> MREDTKVYDITIIGGGPVGLFTAFYGGMRQASVKIIESLPQLGGQLSALYPEKYIYDVAGFPKIRA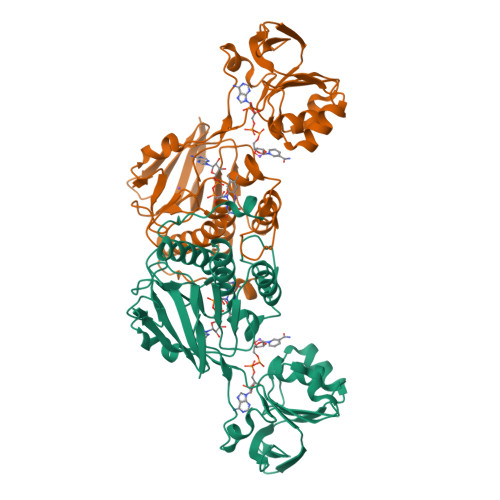QELINNLKEQMAKFDQTICLEQAVESVEKQADGVFKLVTNEETHYSKTVIITAGNGAFKPRKLELENAEQYEGKNLHYFVDDLQKFAGRRVAILGGGDSAVDWALMLEPIAKEVSIIHRRDKFRAHEHSVENLHASKVNVLTPFVPAELIGEDKIEQLVLEEVKGDRKEILEIDDLIVNYGFVSSLGPIKNWGLDIEKNSIVVKSTMETNIEGFFAAGDICTYEGKVNLIASGFGEAPTAVNNAKAYMDPKARVQPLHSTSLFENK>MAKPQVTILATGGTIAGSGESSVKSSYSAGAVTVDKLLAAVPAINDLATIKGEQISSIGSQEMTGKVWLKLAKRVNELLAQKETEAVIITHGTDTMEETAFFLNLTVKSQKPVVLVGAMRSGSSMSADGPMNLYNAVNVAINKASTNKGVVIVMNDEIHAAREATKLNTTAVNAFASPNTGKIGTVYYGKVEYFTQSVRPHTLASEFDISKIEELPRVDILYAHPDDTDVLVNAALQAGAKGIIHAGMGNGNPFPLTQNALEKAAKSGVVVARSSRVGSGSTTQEAEVDDKKLGFVATESLNPQKARVLLMLALTKTSDREAIQKIFSTY[8x]

By administering enzyme drugs called L-asparaginases, which act to quickly deplete Asn in the blood, this drug specifically impacts ALL cells, starving them to death while leaving normal cells largely intact. WoA, like most bacterial Type II L-asparaginases, is a tetramer built by a dimer-of-dimer with 330 residues per protomer. In our structures we observe that the overall fold of each protomer follows the general two-domain fold of bacterial type II L-asparaginases. We sought to clarify this question and to further explain the substrate discrimination, if there is any, between the two forms, by solving the crystal structures of both variants in complex with either the product Asp or L-glutamic acid (Glu).

Each of the four analysed complexes, WoA-P121 + Asp, WoA-P121 + Glu, WoA-S121 + Asp and WoA-S121 + Glu, has in the crystallographic asymmetric unit essentially four (or 8 in the case of WoA-S121 + Glu) identical protomers that build up the corresponding tetramer(s), as shown by very small root mean square deviations of ~0.07 Å; 0.06 Å; 0.07 Å and 0.05 Å, respectively (over 300–330 atoms). Surprisingly, we observed unambiguous electron density for an open conformation of the flexible loop in the other three structures, WoA-P121 + Glu, WoA-S121 + Asp and WoA-S121 + Glu. Moreover, in the WoS121-Glu structure, we observed slight variations in the open loop conformation among the eight protomers of the asymmetric unit. Inspection of the WoA-S121 + Glu and WoA-P121 + Glu structures revealed essentially identical Glu conformations. Except for the side chains of Ser121 versus Pro121, no notable differences were found in the active sites of the two structures. Pro121 brings a ring stacking force along with π-aromatic ring interactions to stabilize Tyr27 in the closed state. In contrast, Ser121 fails to add any additional contribution to assist loop closing on Gln. As a result of the reduced ability of WoA-S121 to achieve the closed/active state with Gln, the L-glutaminase rate (but not Km value) is reduced by ~8-fold related to WoA-P121.> MDEKSTKIIMWLKKMFGDKPLPPYEVNTRTMEILYQLAEWNEARDKDLSLVTEDLKLKSAEVKAEAKYLQDLLTEGLGPSYTNLSRMGNNYLNQIVDSCLALELKNSSLSSYIPAVNDLSSELVAIELNNQEMEAELTSLRKKLTEALVLEKSLERDLKKAEEQCNFEKAKVEIRSQNMKKLKDKSEEYKYKIHAAKDQLSSAGMEEPLTHRSLVSLSET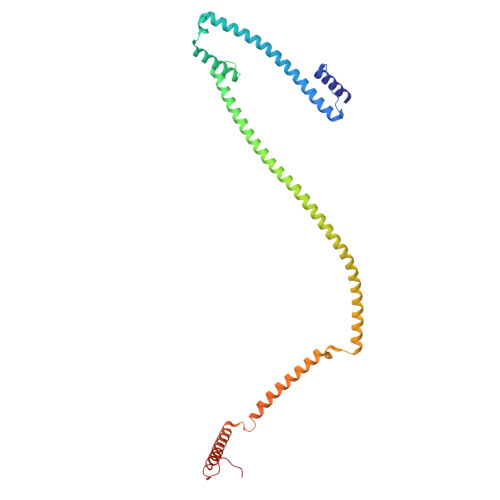LTELKAQSMAAKEKLNSYLDLAPNPSLVKVKIEEAKRELKATEVELTTKVNMMEFVVPEPSKRRLK Mucinases of human gut bacteria cleave peptide bonds in mucins strictly depending on the presence of neighboring O-glycans. The Akkermansia muciniphila AM0627 mucinase cleaves specifically in between contiguous (bis) O-glycans of defined truncated structures, suggesting that this enzyme may recognize clustered O-glycan patches. AM0627 exhibits preference for bis-T over bis-Tn (GalNAcα1-O-Ser/Thr) O-glycopeptide substrates, with the first GalNAc residue being essential for cleavage. AM0627 follows a mechanism relying on a nucleophilic water molecule and a catalytic base Glu residue.

Initially, we chemoenzymatically synthetized a P-selectin glycoprotein ligand 1 (PSGL-1)-like bis-T glycopeptide (hereafter P1 and defined by the sequence TEAQT**T**PPPA in which ** denotes a Galβ1-3GalNAc disaccharide) based on AM0627 substrate cleavage consensus motif determined by a previous mass spectrometry study. The truncated AM0627E326A (P71-E506) enzyme construct produced better diffracting orthorhombic crystals (space group P212121) in the presence of P1 and ZnCl2. The crystal structure of AM0627E326A was solved at 1.9 Å using zinc single-wavelength anomalous dispersion (Zn-SAD; see the “Methods” section). The model obtained from SHELXE26 allowed us to solve the structure of the AM0627E326A–P1–Zn2+ complex at a higher resolution (1.5 Å) by molecular replacement using PHASER27 (see Supplementary Table 1 and see the “Methods” section). The AM0627E326A crystal structure revealed two distinct domains formed by an Ig-like fold domain and the M60-like catalytic domain. In addition, a water molecule did not coordinate the zinc ion and therefore did not replace the role of the P1 Thr5 carbonyl group in coordinating the metal. However interestingly, in our structure, we observed the presence of a potential catalytic water molecule, further discussed below, which was visualized in the active site establishing hydrogen bonds with the Thr5 carbonyl group, the acetamide NH group of the GalNAc located at G1, and the NH group of Thr6 (Fig. 1b for the subsite nomenclature of the sugar moieties and Fig. 2b, c). The Glu2 side chain makes a hydrogen bond with the Asp292 side chain, the Ala3 methyl group establishes CH–π interactions with the side chains of Trp149/Phe290, and Gln4 forms hydrogen bonds with Arg291 (both side chain and backbone). Regarding the two glycosylated Thr residues (Thr5 and Thr6 in Fig. 3a), the Thr5 backbone forms a hydrogen bond with the Tyr470 side chain, the Thr5 methyl group forms a CH–π interaction with the Tyr287 side chain and the Thr6 backbone makes a hydrogen bond with the Tyr287 side chain. Additional enzyme–substrate interactions involve the two contiguous T O-glycans (bis-T) of P1.

>[2x]GGGGGPDYLYAEYRALPSPRQTGKNLRIGDGFSKYDNMTGVYLEKGRHVVLVGKTEGQEISLLLPNLMRKPAEGVQPTKDPNGWGLHKKQIPLKEGINIIDVETPANAYISYFTEDAGKAPKIPVHFVTGKANGYFDTTRGDTNKDWVRLLDQAVSPIMDARGKYIQVAYPVEFLKKFTKDRGTELINAYDKLIGIQYQLMGLDKYGKIPENRVLARVNFNYYMFRDGDGVAYLGNDGTMRMVTDPENVLKGDACWGFSHAVGHVMQMRPMTWGGMTEVSNNIFSLQAAAKTGNESRLKRQGSYDKARKEIIEGEIAYLQSKDVFNKLVPLWQLHLYFTKNGHPDFYPDVMEYLRNNAGNYGGNDTVKYQFEFVKACCDVTKTDLTDFFEKWGFFKPGKFHIGDYAQYDFNVTPEMVEETKKWIAGKGYPKPETDITELSE;>TEAQTTPPPA[2x]> MGSDAFDEMDEIWALYADDGAQALDAMEASLLALQAGEDAAAHVGPLFRAVHTFKGNSRVLGLSVVESRAHLCEDLIGLVRDAGVPMDGEIVEILLFASDTL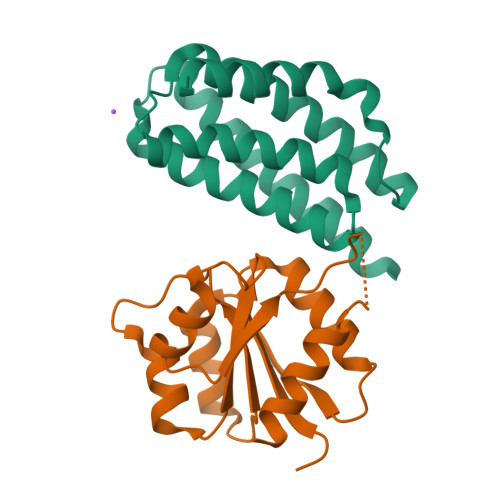RAMLEETAASRADVEGTGSEALMDQLRSKIARCSRSHHHHHH;> MRGSHHHHHHGSPYNVMIVDDAAMMRLYIASFIKTLPDFKVVAQAANGQEALDKLAAQPNVDLILLDIEMPVMDGMEFLRHAKLKTRAKICMLSSVAVSGSPHAARARELGADGVVAKPSGTVSHDLEEKTGGELARTMRTLMAA In this work, we exhaustively probe the ability of all 36 immobile HJ sequences to form DNA crystals in two different designed systems. Three separate self-assembling DNA crystal systems are described in this report: the “4 × 5” and “4 × 6” designs (collectively referred to as the 4 × N systems), and a third construct with a “scrambled” sequence variant of the 4 × 6 lattices. Self-assembly was mediated by three constituent oligonucleotides: (S1) containing four sequence repeats of either 5 or 6 bases; (S2) composed of 21 bases containing complementary regions to both (S1); and (S3) which forms the second junction crossover. The HJ serves as the fundamental component at the core of each unit, and the ultimate assembly of the full lattice is facilitated by the complementary 2-base sticky ends that tail each duplex.

Each asymmetric unit could be defined as either a HJ containing 10 and 11 bp on each arm, or as a 21-bp linear duplex. Both versions were solved in parallel, yielding a total of 134 crystal structures (Supplementary Table 1 for data collection and refinement statistics). The 4 × 5 system robustly crystallized with 75% of the junctions, and we obtained crystals in all but 9 of 36 sequences. Of the resulting structures, 18 exhibited P32 symmetry with average cell dimensions a = b = 68.85 Å c = 60.09 Å, with only nine retaining the original P3221 symmetry with average cell edges a = b = 68.17 Å c = 60.60 Å. Although the cell parameters between the two symmetries were virtually indistinguishable, the differences between the periodicity of the lattices is dramatic, with vastly different cavity sizes. While the highest resolution achieved for the J1 system was 3.1 Å, in roughly half of the crystals measured the resolutions were 3.05 Å or better, and as high as 2.9 Å (J6) and 2.75 Å (J19), for the P32 and P3221 symmetries, respectively.

> GAGCAGACGAG;> ACCCCACTCA;> CTGGT;> TCTGAGTGGCGTCTGC> 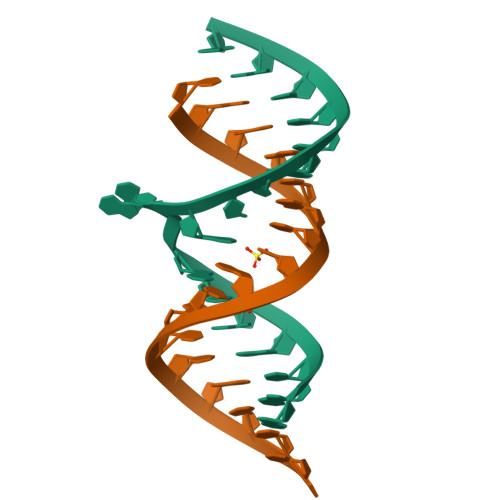GGUGGUGAAGUCGCUCGG;> CGAGCGUCACACCACCC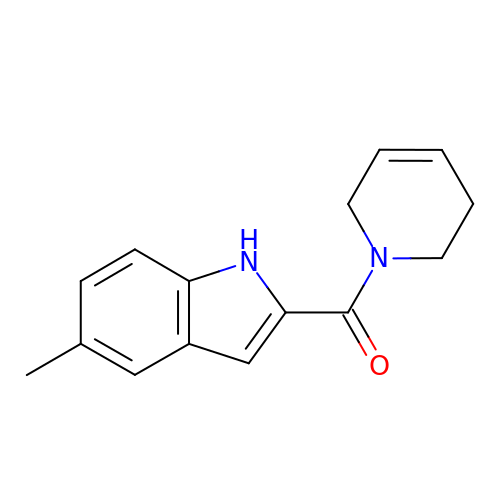3,6-dihydropyridin-1(2H)-yl(5-methyl-1H-indol-2-yl)methanone | C15 H16 N2 O | QRPYFEVBXZYSAL-UHFFFAOYSA-N> MVQAVAVLKGDAGVSGVVKFEQASESEPTTVSYEIAGNSPNAERGFHIQEFGDATNGCVSAGPHFNPFKKTHGAPTDEVRHVGDMGNVKTDENGVAKGSFKDSLIKLIGPTSVVGRSVVIHAGQDDLGKGDTEESLKTGNA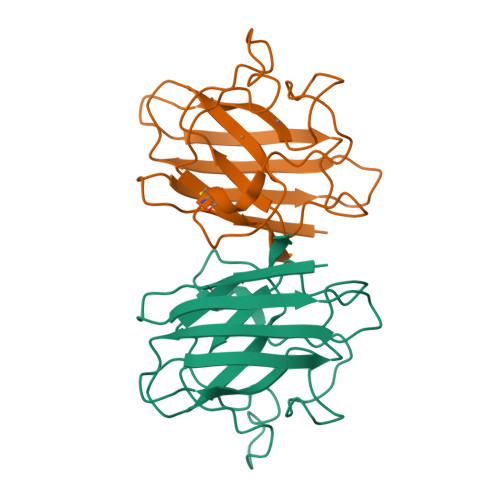GPRPACGVIGLTN> VASLYQAVS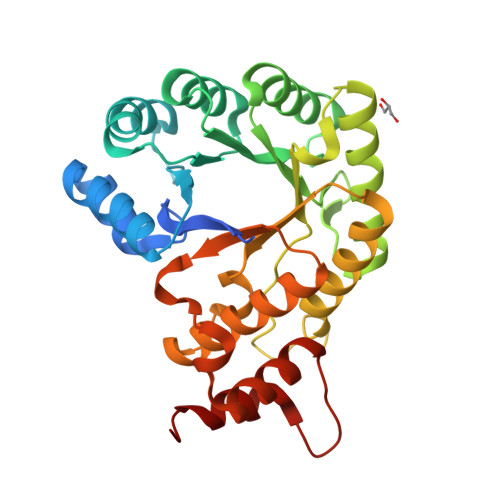LKQEASLFLVGERLNATGSKRFREMLFARDLEGILALAREQVEEGAHALDLSVAWTGRDELEDLRWLLPHLATALTVPVMVDSTSPEAMELALKYLPGRVLLNSANLEDGLERFDRVASLAKAHGAALVVLAIDEKGMAKTREEKVRVALRMYERLTEHHGLRPEDLLFDLLTFPITQGDEESRPLAKETLLAMEELRERLPGVGFVLGVSNVSFGLKPRARRVLNSVFLDEARKRGLTAAIVDAGKILPISQIPEEAYALALDLIYDRRKEGFDPLLAFMAYFEAH>APAAVDWRARGAVTAVKDQGQCGSCWAFSAIGNVECQWFLAGHPLTNLSEQMLVSCDKTDSGCSGGLMNNAFEWIVQENNGAVYTEDSYPYASGEGISPPCTTSGHTVGATITGHVELPQDEAQIAAWLAVNGPVAVAVDASSWMT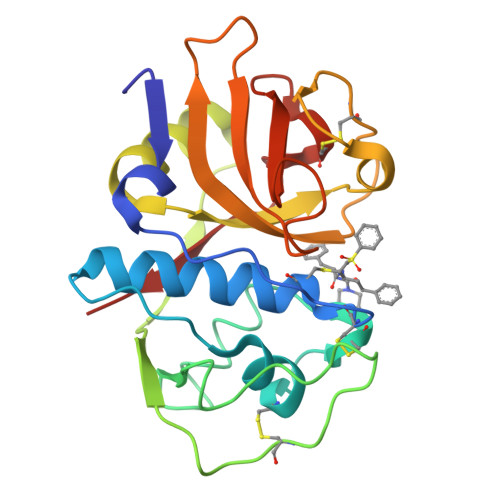YTGGVMTSCVSEQLDHGVLLVGYNDSAAVPYWIIKNSWTTQWGEEGYIRIAKGSNQCLVKEEASSAVVG[3x]>GIEDLIDTAIKNALRVSQPPSTQSTEATSGVNSQEVPALTAVETGASGQAIPSDVVETRHVVNYKTRSESCLESFFGRAACVTILSLTNSSKSGEEKKHFNIWNITYTDTVQLRRKLEFFTYSRFDLEMTFVFTENYPSTASGEVRNQVYQIMYIPPGAPRPSSWDDYTWQSSSNPSIFYMYGNAPPRMSIPYVGIANAYSHFYDGFARVPLEGENTDAGDTFYGLVSINDFGVLAVRAVNRSNPHTIHTSVRVYMKPKHIRCWCPRPPRAVLYRGEGVDMISSAILPLAKVDSITTF[5x];>[5x]SPNVEACGYSDRVRQITLGNSTITTQEAANAIVAYGEWPTYINDSEANPVDAPTEPDVSSNRFYTLESVSWKTTSRGWWWKLPDCLKDMGMFGQNMYYHYLGRSGYTIHVQCNASKFHQGALGVFLIPEFVMACNTESKTSYVSYINANPGERGGEFTNTYNPSNTDASEGRKFAALDYLLGSGVLAGNAFVYPHQIINLRTNNSATIVVPYVNSLVIDCMAKHNNWGIVILPLAPLAFAATSSPQVPITVTIAPMCTEFNGLRNITVPVHQ;>[5x]GLPTMNTPGSNQFLTSDDFQSPCALPNFDVTPPIHIPGEVKNMMELAEIDTLIPMNAVDGKVNTMEMYQIPLNDNLSKAPIFCLSLSPASDKRLSHTMLGEILNYYTHWTGSIRFTFLFCGSMMATGKLLLSYSPPGAKPPTNRKDAMLGTHIIWDLGLQ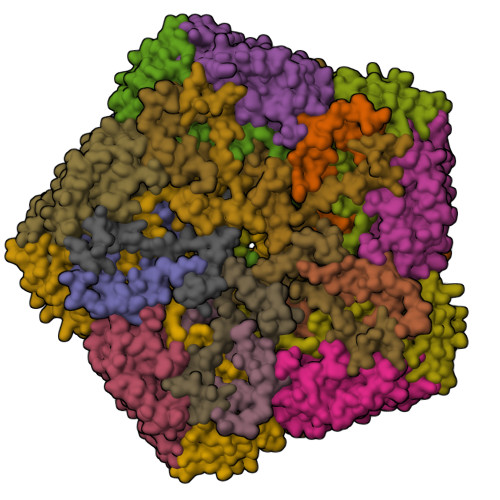SSCSMVAPWISNTVYRRCARDDFTEGGFITCFYQTRIVVPASTPTSMFMLGFVSACPDFSVRLLRDTPHISQSKLIGRTQ;>[5x]MGAQVSTQKTGAHENQNVAANGSTINYTTINYYKDSASNSATRQDLSQDPSKFTEPVKDLMLKTAPALN Here, we report the structure and kinetic rate parameters for a glycoside hydrolase (GH) family 5 subfamily 4 enzyme (CelD) from Piromyces finnis, a modular, cellulosome-incorporated endoglucanase that possesses three GH5 domains followed by two C-terminal fungal dockerin domains (double dockerin). In this study, we characterized, at the structural and functional levels, the CelD enzyme from the anaerobic fungus Piromyces finnis. This fungal enzyme belongs to the glycoside hydrolase (GH) family 5 subfamily 4 of cellulases and acts strictly as an endo-β-1,4-glucanase (EC 3.2.1.4) with confirmed activity against carboxymethylcellulose (CMC), mixed linkage glucan (MLG), and xyloglucan. The CelD catalytic domain displays strong structural similarity to GH clan A, a group of 28 unique GH families exhibiting a (β/α)8–barrel fold in structure, with the highest sequence similarity to proteins from GH5 subfamily 4 (GH5_4), a family of enzymes that predominantly display endoglucanase activity (EC 3.2.1.4). Like other GH5 enzymes, CelD contains two invariant catalytic glutamate residues, the acid/base Glu154 and the nucleophile Glu278.

To facilitate bacterial protein expression and to study the contribution of fungal dockerins to enzyme catalytic activity, we characterized a single GH5 catalytic domain in isolation (ORX48147.1 residues 748–1105), as well as a GH5 with the native C-terminal double dockerin (ORX48147.1 residues 748–1192) and a GH5 with native C-terminal double dockerin and a non-native N-terminal dockerin domain. We present the crystal structure of a CelD GH5 catalytic domain in its apo wild-type form and complementary structure of an inactive E154A mutant in complex with cellotriose solved at a resolution of 2.5 Å and 1.8 Å, respectively (for convenience, in this work, we used 1–362 numbering for the catalytic domain which corresponds to 91–452 residue numbering of the “1–536” in Supplemental Table S1). The crystals of the apo form and the complex belonged to orthorhombic P212121 space group and contained two domain molecules per asymmetric unit. Almost all amino acid residues of the CelD catalytic domain, with the exception of a few side chains and three C-terminal residues, were traceable in the final electron density map. Structural features that differentiated the P. finnis catalytic domain from other GH5 enzymes were longer loops around the substrate binding site (between βI/α1, βIV/α4, α5/βVI, and βVIII/α8) and possessing only one disulfide bridge instead of four present in GH5’s from other fungi. The overall root mean square deviation (RMSD) between apo wild form and inactive E154A-ligand complex protein models was 0.26 Å for 359/362 Cα pairs, demonstrating high overall similarity and illustrating that substrate binding results in little to no conformational change. We did not observe substantial conformational changes between the apo-enzyme structure and the mutant structure with the bound ligand.

>[2x]SNAIRDISSIELIKEMRFGWNLGNTLDAECTSWMDYEKNPIGSETCWGNVKTNEDIFKTLMDNQFNVFRIPTTWTGHIGEAPEYKINEQWMKRVHEIVDYPYKNGAFVILNIHHETWNHAFAETVDEAKVELAQVWKQIAEEFKGYGERLIFEGQNEPRKNGTPVEWNGGDKEGWDVVNAMNAVFLETVRSSGGNNAKRHLMIPPYAAACNENSFKNFDFPEDDDKVIASVHAYSPYNFALNNGEGAVDKFDASGKNELDWNINLMKKRFVDQGIPMILGEYGAMNRDNEEERAAWAEYYMEKITALGVPQVWWDNGVFEGEGERFGLIDRKNLKIVYPSIVAALQKGRGLEVNVLHAIETEPEE>[2x]SMCLKLNLLDHVFANPFMNAAGVLC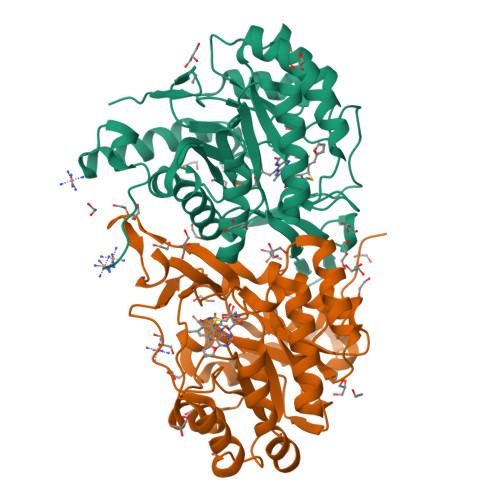STEEDLRCMTASSSGALVSKSCTSAPRDGNPEPRYMAFPLGSINSMGLPNLGFDFYLKYASDLHDYSKKPLFLSISGLSVEENVAMVRRLAPVAQEKGVLLELNLSCPNVPGKPQVAYDFEAMRTYLQQVSLAYGLPFGVKMPPYFDIAHFDTAAAVLNEFPLVKFVTCVNSVGNGLVIDAESESVVIKPKQGFGGLGGKYILPTALANVNAFYRRCPDKLVFGCGGVYSGEDAFLHILAGASMVQVGTALQEEGPGIFTRLEDELLEIMARKGYRTLEEFRGRVKTIE> SMDDDQVAFSFILDNIVTQKMMAVPDSWPFHHPVNKKFVPDYYKVIVNPMDLETIRKNISKHKYQSRESFLDDVNLILANSVKYNGPESQYTKTAQEIVNVCYQTLTEYDEHL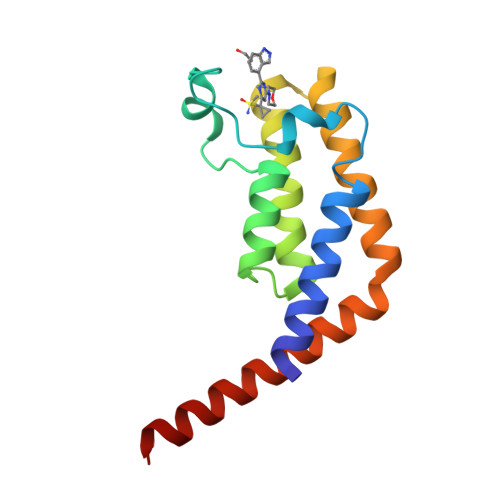TQLEKDICTAKEAALEEAELESLD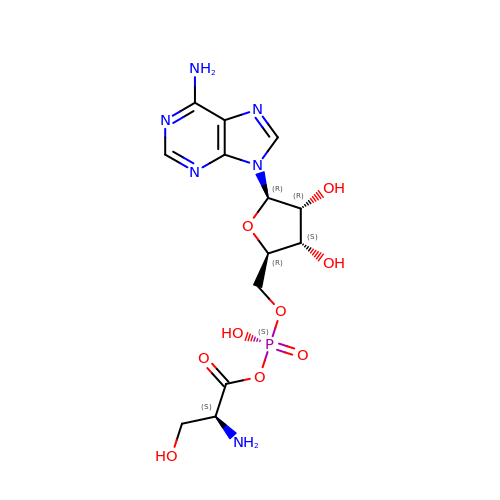SERYL ADENYLATE | C13 H19 N6 O9 P | UVSYURUCZPPUQD-MACXSXHHSA-N> S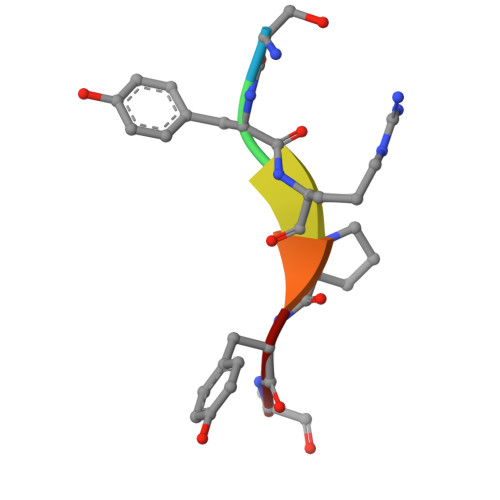YRPYA>[9x]MNAKEIVVHALRLLENGDARGWSDLFHPEGVLEYPYPPPGYKTRFEGRETIWAHMRLFPEYMTIRFTDVQFYETADPDLAIGEFHGDGVLTA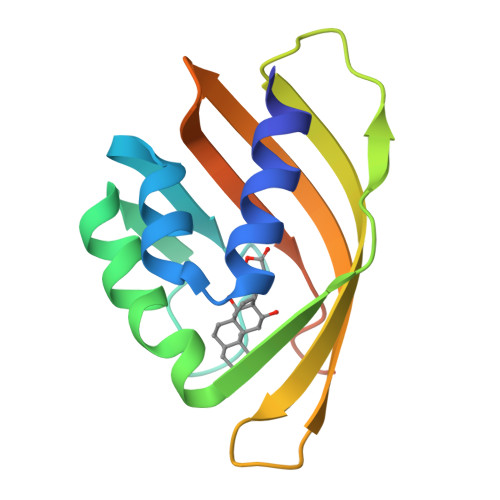SGGKLAYDYIAVWRTRDGQILLYRLFFNPLRVLEPLGLEHHHHHH(+)cis-chlordane 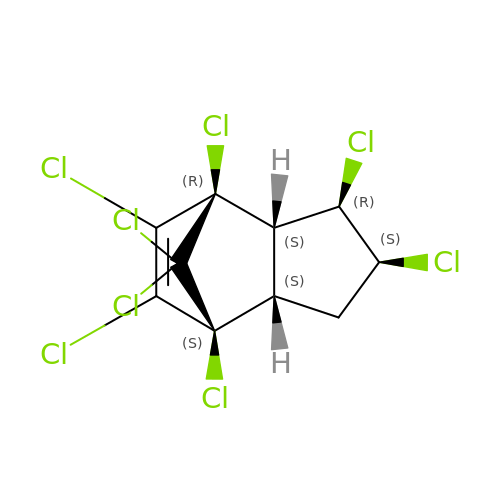| C10 H6 Cl8 | BIWJNBZANLAXMG-KMMBHOGFSA-N The circadian clock of the cyanobacterium Synechococcus elongatus can be reconstituted in vitro by three proteins, KaiA, KaiB and KaiC. Homo-hexameric KaiC displays kinase, phosphatase and ATPase activities; KaiA enhances KaiC phosphorylation and KaiB antagonizes KaiA. The crystal structure of KaiC from S. elongatus revealed a hexamer in the shape of a double doughnut with approximate dimensions 100×100 Å, whereby the N-terminal CI and C-terminal CII halves of subunits are joined by a 15-amino acid linker. Two phosphorylation sites (P-sites), T432 and S431 that are both located in the CII half were identified in KaiC.

To analyze the phosphorylation patterns of KaiC P-site mutants and to visualize potential conformational variations in the vicinity of bound ATP and residues 432 and 431 at hexamer subunit interfaces, we determined crystal structures of the S. elongatus KaiC single mutants T432A (TSa), S431A (TaT), S431D (TdT), and T426N (nST) and the double mutants T426A/T432A (aSa) and S431A/T432E (Tae). b KaiC mutations xyz or mutants KaiCxyz are sequentially shown in order of sites x = 426, y = 431, and z = 432 where the wild-type residue is in upper case and mutated residues are shown in lower case, i.e. Tsa or KaiCTSa, where the residue at position 426 is T, the residue at position 431 is S, and the residue at position 432 is mutated to A. The structures of the TdT, nST and aSa mutants provide further support for the conclusion that T432 is the principal phosphorylation site because it lies closest to the γ-phosphate. The combined structural data expose subtle changes in the orientations of the H423-I433 loop region harboring phosphorylated residues relative to the γ-phosphate of ATP compared with the structure of wt-KaiC.

>MTSAEMTSPNNNSEHQAIAKMRTMIEGFDDISHGGLPIGRSTLVSGTSGTGKTLFSIQFLYNGIIEFDEPGVFVTFEETPQDIIKNARSFGWDLAKLVDEGKLFILDASPDPEGQEVVGGFDLSALIERINYAIQKYRARRVSIDSVTSVFQQYDASSVVRRELFRLVARLKQIGATTVMTTERIEEYGPIARYGVEEFVSDNVVILRNVLEGERRRRTLEILKLRGTSHMKGEYPFTITDHGINIFPLGAMRLTQRSSNVRVSSGVVRLDEMCGGGFFKDSIILATGATGTGKTLLVSRFVENACANKERAILFAYEESRAQLLRNAYSWGMDFEEMERQNLLKIVCAYPESAGLEDHLQIIKSEINDFKPARIAIDSLSALARGVSNNAFRQFVIGVTGYAKQEEITGLFTNTSDQFMGAHSIADSHISAITDTIILLQYVEIRGEMSRAINVFKMRGSWHDKAIREFMISDKGPDIKDSFRNFERIISGSPTRITVDEKSELSRIVRGVQEKGPES[6x]>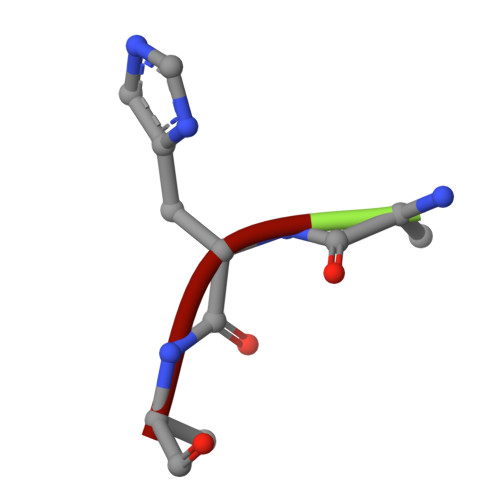 AHA>[2x]MGSSHHHHHHSSGLVPRGSHMTDLSDVSRTAAAKPPAVPGRGPANKVRFVTAASLFDGHDASINIMRRILQSQGCEVIHLGHNRSVQEVVTAALQEDVQGIAISSYQGGHVEYFKYMIDLLREHGGEHIQVFGGGGGVIVPDEIRELQAYGVARIYSPEDGQRMGLAGMITDMAQRCDIDLTRYAPTTLDTVVAGDRRALAQLITALENGKADPELVSALHAQAKAAAVPVLGITGTGGAGKSSLTDELIRRFRLDQDDALSIAVISIDPSRRKSGGALLGDRIRMNAINHPNIFMRSLATREAGSEISQALPDVIAACKAARFDLVIVETSGIGQGDAAIVPHVDLSLYVMTPEFGAASQLEKIDMLDFADFVAINKFDRKGAQDAWRDVAKQVQRNREQWHSRAEDMPVYGTQASRFNDDGVTMLYQGLVGALGARGMSLKPGTLPNLEGRISTGQNVIVPPARSRYLAELADTVRAYHRRVVAQSKLARERQQLRAAHDMLQGAGHESAALETLASERDVSLGAVERKLLAMWPQMQQAYSGDEYVVKIRDKEIRTGLISTTLSGTKIRKVVLPRFEDEGEILKWLMRENVPGSFPYTAGVFAFKREGEDPTRMFAGEGDAFRTNRRFKLVSEGMEAKRLSTAFDSVTLYGEDPHERPDIYGKVGNSGVSIATLEDMKVLYDGFDLTNPSTSVSMTINGPAPTILAMFMNTAIDQQIDRFRADNGRDPTADEEAKIRAWVLQNVRGTVQADILKEDQGQNTCIFSTEFSLKVMGDIQEYFVHHQVRNFYSVSISGYHIAEAGANPISQLAFTLANGFTYVEAYLARGMHIDDFAPNLSFFFSNGMDPEYSVLGRVARRIWAVTMRDKYGANDRSQKLKYHIQTSGRSLHAQEIDFNDIRTTLQALIAIYDNCNSLHTNAYDEAITTPTAESVRRALAIQLIINREWGVAKCENPNQGSFLIEELTDLVEEAVLQEFERIAERGGVLGAMETGYQRGKIQEESLYYEQLKHDGTLP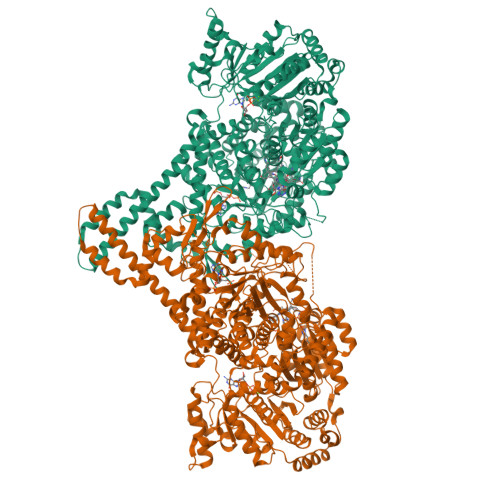IIGVNTFRNPNGDPTPQTLELARSSEDEKQSQLHRLTEFHGAHQADAEAMLARLRQAVIDNRNVFAVLMDAVRVCSLGQITHALFEVGGQYRRNM>MAANSTRRPIIAFMSDLGTTDDSVAQCKGLMYSIC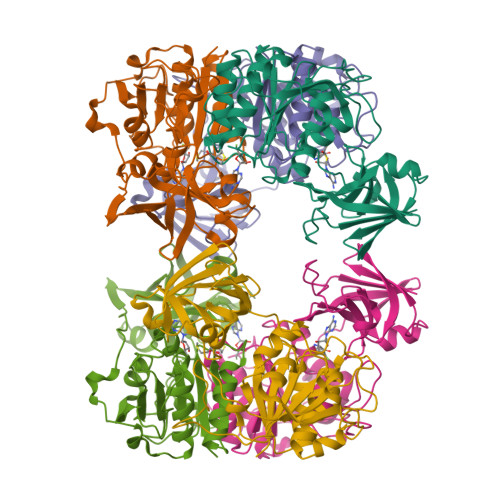PDVTVVDVCHSMTPWDVEEGARYIVDLPRFFPEGTVFATTTYPATGTTTRSVAVRIKQAAKGGARGQWAGSGAGFERAEGSYIYIAPNNGLLTTVLEEHGYLEAYEVTSPKVIPEQPEPTFYAREMVAIPSAHLAAGFPLSEVGRPLEDHEIVRFNRPAVEQDGEALVGVVSAIDHPFGNVWTNIHRTDLEKAGIGYGARLRLTLDGVLPFEAPLTPTFADAGEIGNIAIYLNSRGYLSIARNAASLAYPYHLKEGMSARVEAR[3x]> GAMAAPAACTRFSDNYDIKEELGKG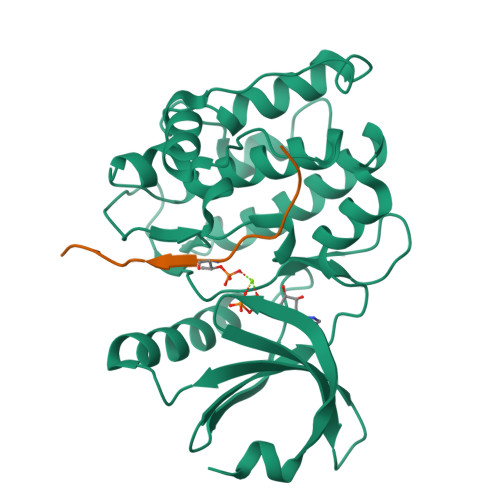AFSIVKRCVQKSTGFEFAAKIINTKKLTARDFQKLEREARICRKLHHPNIVRLHDSIQEENYHYLVFDLVTGGELFEDIVAREFYSEADASHCIQQILESVNHCHQNGVVHRNLKPENLLLASKAKGAAVKLADFGLAIEVQGDHQAWFGFAGTPGYLSPEVLKKEPYGKSVDIWACGVILYILLVGYPPFWDEDQHRLYSQIKAGAYDYPSPEWDTVTPEAKNLINQMLTVNPNKRITAAEALKHPWICQRERVASVVH;> GVLPKAPKLQASQATLARQDTIDEGGEVDSSPPSRDSRVVIEGAAVSSATVGPS> EPQVLCYLTSWSSKRPSAGRFMPENVDPTLCTHVIYAFATLKDHKLTEADEKDADMYDKVVALREKNPNLKILLAIGGWAFGSTPFKELTSNVFRMNQFVYEAIEFLRDYQFNGLDVDWLYPRGADDRAAFVSLLKELRLAFEGEAKTSGQPRLLLTAAVPASFEAIAAGYDVPEISKYLDFINVMTYDFHGQWERQVGHNSPLFPLESATSYQKKLTVDYSAREWVRQGAPKEKLMIGMPTYGRSFTLINDTQFDIGAPASGGGQAGRFTNEAGFMSYYEICEFLREDNTTLVWDNEQMVPFAYREDQWVGFDDERSLKTKMAWLKEEGFGGIMVWSVDMDDFRGSCGTGKYPLITAMKQELSGYKVKLEYDGPYESSSPTGQYTTKDPHEVTCEEEDGHISYHKDHADCTMYYMCEGERKHHMPCPSNLVFNPNENVCDWPENVEGCQQHTQAPAAKR

Here, we report an arthropod-conserved insect chitinase belonging to group III from the pest Ostrinia furnacalis (OfChtIII), which contains two GH18 domains that act without synergism according to enzymatic assays and structural investigations. OfChtIII contains 987 amino-acid residues and is composed of four domains: a predicted TM domain (residues 7–29), two catalytic domains, GH18A (residues 94–461) and GH18B (residues 530–889), and a CBM14 domain (residues 922–976). The two GH18 domains of OfChtIII possess similar structures and substrate specificities, which differentiate them from the chitinolytic chitinase OfChtI-CAD. The degradation activity of GH18A and GH18B (or GH18B-CBM14) in combination towards EGC was equal to the activity calculated from the sum of the individual activities, suggesting that there was no synergistic effect between them.

To study the substrate-binding mode, the structures of two complexes of GH18B were crystallized and obtained: that of wild-type GH18B complexed with (GlcNAc)3 and that of the GH18B-E647L mutant with a bound (GlcNAc)5.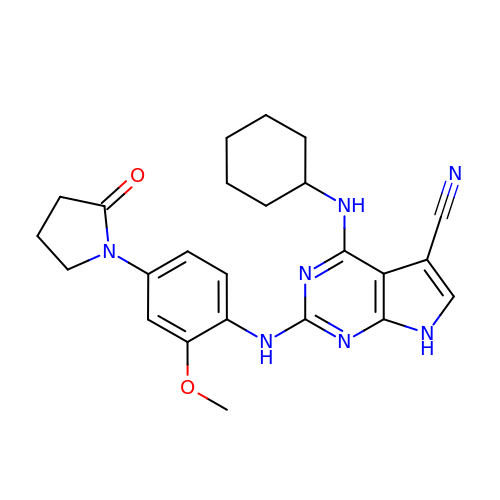4-(cyclohexylamino)-2-[[2-methoxy-4-(2-oxidanylidenepyrrolidin-1-yl)phenyl]amino]-7H-pyrrolo[2,3-d]pyrimidine-5-carbonitrile | C24 H27 N7 O2 | LOHMGKJWMIIPRA-UHFFFAOYSA-N>PVFSADPGAPAPVNPCCYYPCQHQGICVRFGLDRYQCDCTRTGYSGPNCTIPEIWTWLRTTLRPSPSFIHFLLTHGRWLWDFVNATFIRDTLMRLVLTVRSNLIPSPPTYNIAHDYISWESFSNVSYYTRILPSVPRDCPTPMGTKGKKQLPDAEFLSRRFLLR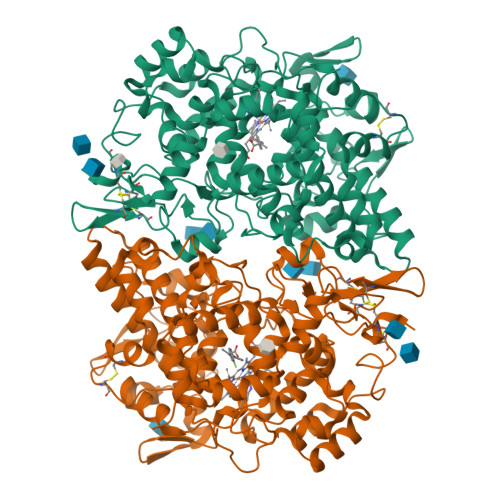RKFIPDPQGTNLMFAFFAQHFTHQFFKTSGKMGPGFTKALGHGVDLGHIYGDNLERQYQLRLFKDGKLKYQMLNGEVYPPSVEEAPVLMHYPRGIPPQSQMAVGQEVFGLLPGLMLYATIWLREHNRVCDLLKAEHPTWGDEQLFQTARLILIGETIKIVIEEYVQQLSGYFLQLKFDPELLFGAQFQYRNRIAMEFNQLYHWHPLMPDSFRVGPQDYSYEQFLFNTSMLVDYGVEALVDAFSRQPAGRIGGGRNIDHHILHVAVDVIKESRVLRLQPFNEYRKRFGMKPYTSFQELTGEKEMAAELEELYGDIDALEFYPGLLLEKCHPNSIFGESMIEMGAPFSLKGLLGNPICSPEYWKASTFGGEVGFNLVKTATLKKLVCLNTKTCPYVSFHVPDPRQEDRPGVERPPTEL[2x]>[2x]MDAATTRVGLTDLTFRLLRESFADAVSWVAKNLPARPAVPVLSGVLLTGSDNGLTISGFDYEVSAEAQVGAEIVS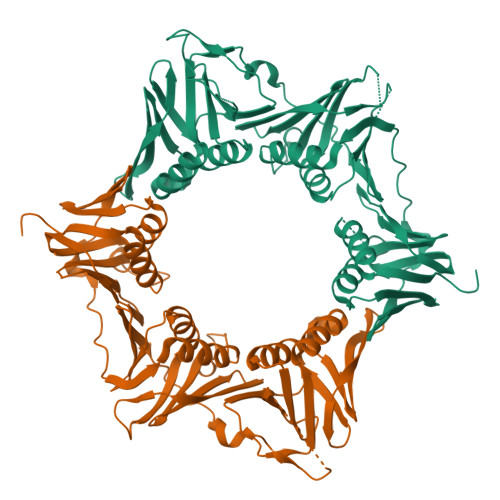PGSVLVSGRLLSDITRALPNKPVDVHVEGNRVALTCGNARFSLPTMPVEDYPTLPTLPEETGLLPAELFAEAISQVAIAAGRDDTLPMLTGIRVEILGETVVLAATDRFRLAVRELKWSASSPDIEAAVLVPAKTLAEAAKAGIGGSDVRLSLGTGPGVGKDGLLGISGNGKRSTTRLLDAEFPKFRQLLPTEHTAVATMDVAELIEAIKLVALVADRGAQVRMEFADGSVRLSAGADDVGRAEEDLVVDYAGEPLTIAFNPTYLTDGLSSLRSERVSFGFTTAGKPALLRPVSGDDRPVAGLNGNGPFPAVSTDYVYLLMPVRLPG> MDLTVEPNLHSLITSTTHKWIFVGGKGGVGKTTSSCSIAIQMALSQPNKQFLLISTDPAHNLSDAFGEKFGKDARKVTGMNNLSCMEIDPSAALKDMNDMAVSRANNNGSDGQGDDLGSLLQGGALADLTGSIPGIDEALSFMEVMKHIKRQEQGEGETFDTVIFD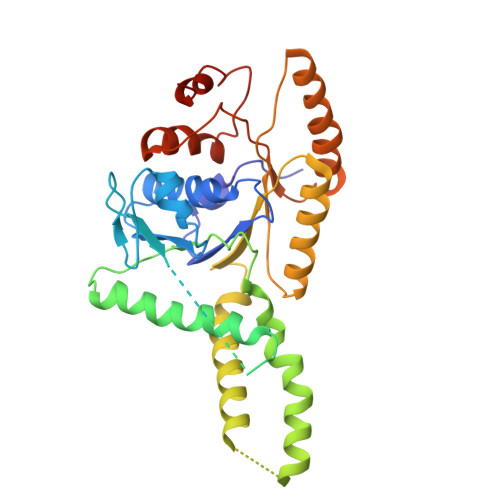TAPTGHTLRFLQLPNTLSKLLEKFGEITNKLGPMLNSFMGAGNVDISGKLNELKANVETIRQQFTDPDLTTFVCVCISEFLSLYETERLIQELISYDMDVNSIIVNQLLFAENDQEHNCKRCQARWKMQKKYLDQIDELYEDFHVVKMPLCAGEIRGLNNLTKFSQFLNKEYNPITDGKVIYELEDKELEHHHHHH> GSKMAFTLADRVTEEMLADKAALVVEVVEENYHDAPIVGIAVVNEHGRFFLRPETALADPQFVAWLGDETKKKSMFDSKRAAVALKWKGIELCGVSFDLLLAAYLLDPAQGVDDVAAAAKMKQYEAVRPDEAVYGKGAKRAVPDEPVLAEHLVRKAAAIWELERPFLDELRRNEQDRLLVELEQPLSSILAEMEFAGVKVDTKRLEQMGKELAEQLGTVEQRIYELAGQEFNINSPKQLGVILFEKLQLPVLKKTKTGYSTSADVLEKLAPYHEIVENILHYRQLGKLQSTYIEGLLKVVRPDTKKVHTIFNQALTQTGRLSSTEPNLQNIPIRLEEGRKIRQAFVPSESDWLIFAADYSQIELRVLAHIAEDDNLMEAFRRDLDIHTKTAMDIFQVSEDEVTPNMRRQAKAVNFGIVYGISDYGLAQNLNISR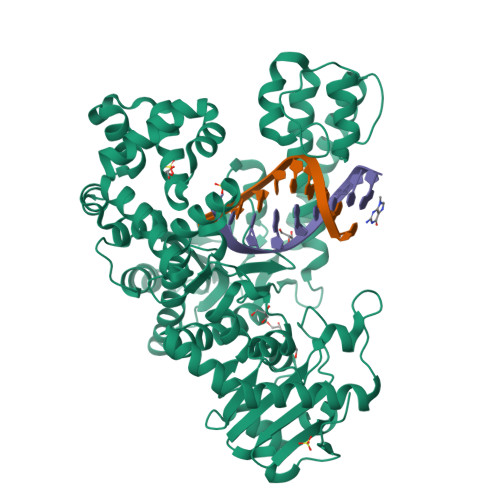KEAAEFIERYFESFPGVKRYMENIVQEAKQKGYVTTLLHRRRYLPDITSRNFNVRSFAERMAMNTPIQGSAADIIKKAMIDLNARLKEERLQAHLLLQVHDELILEAPKEEMERLCRLVPEVMEQAVTLRVPLKVDYHYGSTWYDAK>[4x]EHNFNVVINA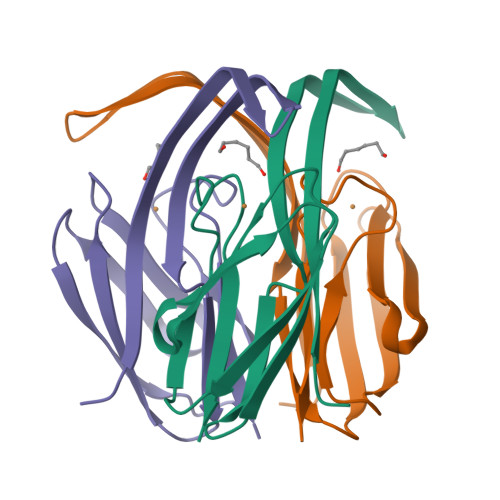YDTTIPELNVEGVTVKNIRAFNVLNEPETLVVKKGDAVKVVVENKSPISEGFSIDAFGVQEVIKAGETKTISFTADKAGAFTIWCQLHPKNIHLPGTLNVVE C. glutamicum is a Gram-positive bacterium that finds industrial use in the production of vitamins and amino acids, including glutamic acid, which is used in the production of the flavoring agent monosodium glutamate. DapE is involved in producing l-lysine and l,l-2,6-diaminopimelate and its catalytic mechanism is likely to involve two zinc ions. The crystal structure of Cgl1109 reveals a dimeric structure from crystal-packing considerations and as also suggested by the PDBePISA server. The dimeric assembly is promoted by the smaller of the two domains of the molecule, while the larger domain is the putative catalytic domain.

Here, we present an independent structure determination of Cgl1109 at ∼3 Å resolution without use of the previous Rosetta model and molecular-replacement solution. The diffraction data for the Cgl1109 crystal structure were quite anisotropic and the effective overall B factors along the principal axes of the unit cell ranged from 60 to 110 Å2. The relatively high anisotropy and high B factors made the structure determination considerably more challenging than for many other structures at a similar resolution of about 3 Å. For Cgl1109, DEN refinement resulted in a model that is closer to the true structure, producing improved model phases that in turn provide a better starting point for automated model building. The improved model phases also provided more significant peaks in anomalous difference Fourier maps to better locate the six selenium sites of the protein. There were several regions that required correction of register shifts and rebuilding of α-­helices that were not corrected even in the second round of DEN refinement and automated model building. The final refinement employed residues 10–369 of Cgl1109 (a 369-residue protein) and other solvent molecules (one phosphate ion and one chloride ion). It was performed against diffraction data collected at the high-energy remote wavelength. c maps initially suggested the possible presence of two zinc ions in the putative catalytic site, which would be expected owing to the addition of 6 mM ZnCl2 during cocrystallization (which was added based on putative functional annotation and ligand screening in a fluorescence-based thermal shift assay). However, we did not model zinc ions in the final model owing to the uncertainty associated with high B factors and the absence of significant peaks in the anomalous difference Fourier maps, including from diffraction data collected at the zinc absorption edge.

> GMNSNQPGLDLLGDPIVLTQRLVDIPSPSGQEKQIADEIEDALRNLNLPGVEVFRFNNNVLARTNRGLASRVMLAGHIDTVPIADNLPSRVEDGIMYGCGTVDMKSGLAVYLHTFATLATSTELKHDLTLIAYECEEVADHLNGLGHIRDEHPEWLAADLALLGEPTGGWIEAGCQGNLRIKVTAHGVRAHSARSWLGDNAMHKLSPIISKVAAYKAAEVNIDGLTYREGLNIVFCESGVANNVIPDLAWMNLNFRFAPNRDLNEAIEHVVETLELDGQDGIEWAVEDGAGGALPGLGQQVTSGLIDAVGREKIRAKFGWTDVSRFSAMGIPALNFGAGDPSFAHKRDEQCPVEQITDVAAILKQYLSE>MNPYIYLGGAILAEVIGTTLMKFSEGFTRLWPSVGTIICYCASFWLLAQTLAYIPTGIAYAIWSGVGIVLISLLSWGFFGQRLDLPAIIGMML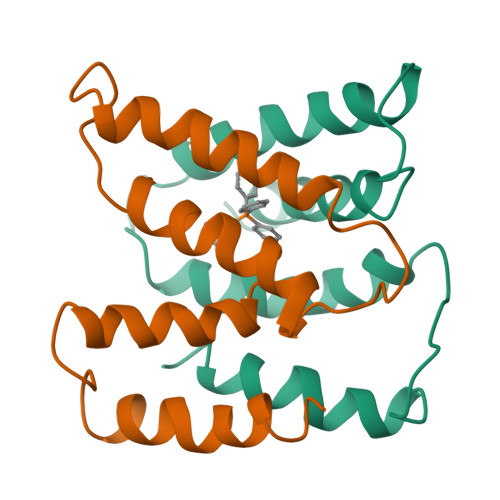ICAGVLIINLLSRSTPH[2x]di(piperidin-1-yl)methanone | C11 H20 N2 O | 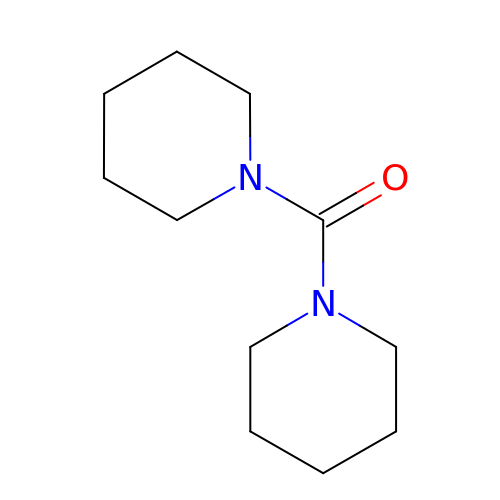SNOJOKOVTYPHMC-UHFFFAOYSA-N>MKSNSQNEKNGSETTNAVGNRKSVTVIGLGPMGQAMADVFLEYGYSVTVWNRTSSKADQLVAKGAIRVSTVNEALAANELVILSLTDYNVMYSILEPVSENLFGKVLVNLSSDTP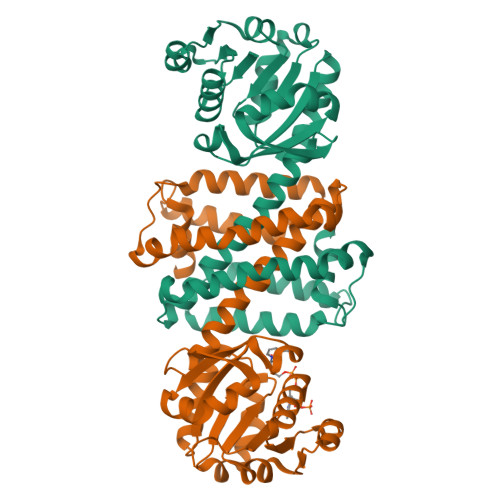EKARKAAKWLEDRGARHITGGVQVPPSGIGKSESYTYYSGDRVVFEAHRETLEVLTSSDYRGEDPGLAMLYYQIQMDIFWTAMLSYLHALAIANANGITAEQFLPYASAMMSSLPKFVEFYTPRLDEGEHPGDVDRLAMGLASVEHVVHTTQEAGIDIALPATVLEVFRRGMKTGHASDSFTSLIEIFKNSDIRS[2x]>[4x]MTRQMILAVGQQG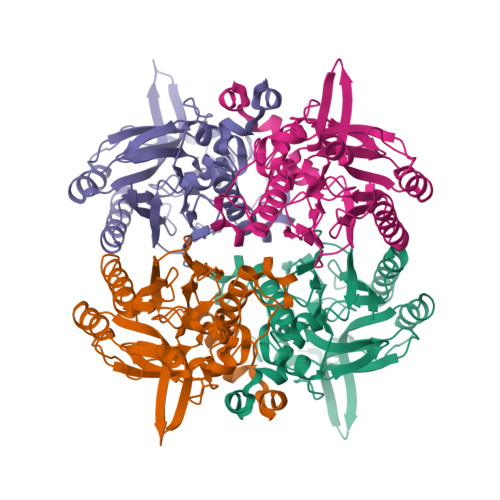PIARAETREQVVGRLLDMLTNAASRGVNFIVFPELALTTFFPRWHFTDEAELDSFYETEMPGPVVRPLFETAAELGIGFNLGYAELVVEGGVKRRFNTSILVDKSGKIVGKYRKIHLPGHKEYEAYRPFQHLEKRYFEPGDLGFPVYDVDAAKMGMFICNDRRWPETWRVMGLKGAEIICGGYNTPTHNPPVPQHDHLTSFHHLLSMQCGSYQNGAWSAAAGKVGMEEGCMLLGHSCIVAPTGEIVALTTTLEDEVITAALDLDRCRELREHIFNFKAHRQPQHYGLIAEF>SRPLSDQEKRKQISVRGLAGVENVTELKKNFNRHLHFTLVKDRNVATPRDYYFALAHTVRDHLVGRWIRTQQHYYEKDPKRIYYLSLEFYMGRTLQNTMVNLALENACDEATYQLGLDMEELEEIEEDAGLGNGGLGRLAACFLDSMATLGLAAYGYGIRYEFGIFNQKICGGWQMEEADDWLRYGNPWEKARPEFTLPVHFYGRVEHTSQGAKWVDTQVVLAMPYDTPVPGYRNNVVNTMRLWSAKAPNDFNLKDFNVGGYIQAVLDRNLAENISRVLYPNDNFFEGKELRLKQEYFVVAATLQDIIRRFKSSKFGCRDPVRTNFDAFPDKVAIQLNDTHPSLAIPELMRVLVDLERLDWDKAWEVTVKTCAYTNHTVLPEALERWPVHLLETLLPRHLQIIYEINQRFLNRVAAAFPGDVDRLRRMSLVEEGAVKRINMAHLCIAGSHAVNGVARIHSEILKKTIFKDFYELEPHKFQNKTNGITPRRWLVLCNPGLAEIIAERIGEEYISDLDQLRKLLSYVDDEAFIRDVAKVKQENKLKFAAYLEREYKVHINPNSLFDVQVKRIHEYKRQLLNCLHVITLYNRIKKEPNKFVVPRTVMIGGKAAPGYHMAKMIIKLITAIGDVVNHDPVVGDRLRVIFLENYRVSLAEKVIPAADLSEQISTAGTEASGTGNMKFMLNGALTIGTMDGANVEMAEEAGEENFFIFGMRVEDVDRLDQRGYNAQEYYDRIPELRQIIEQLSSGFFSPKQPDLFKDIVNMLMHHDRFKVFADYEEYVKCQERVSALYKNPREWTRMVI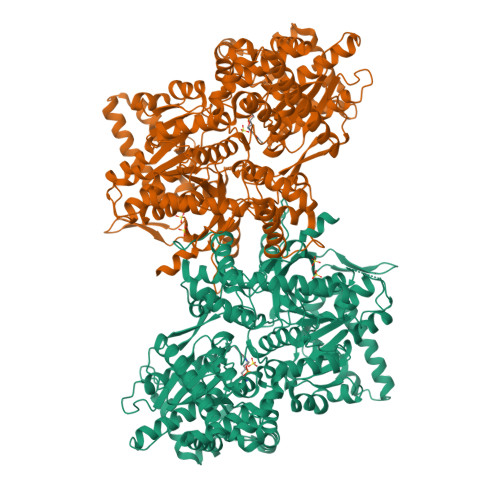RNIATSGKFSSDRTIAQYAREIWGVEPSRQRLPAPDEKIP[4x]>[2x]HHHHHHSSGLVPRGSHMQTTTVYSLEDLLPYLKQDNVDVKLAPGTYNVNGFDVGEDRLFSTTPLFLFEGSNSTYDFTDVKLNINTVVLTKFGNNEVNEIQILGNNNVLKNLKLEDIGTTAPSNRAQSIVIDGRDNRIEG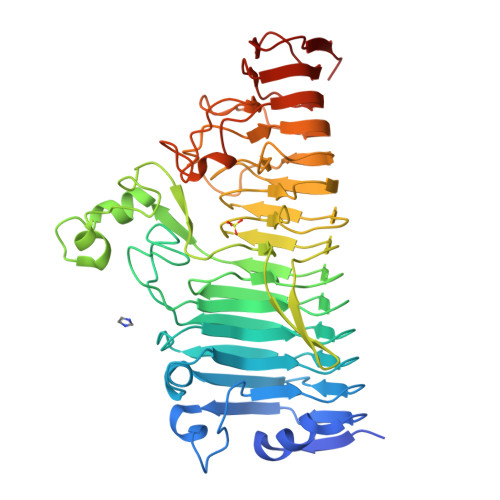FHLTIRGSYPYGYGDAFGKGGGSVINHRKHSGVLIRGLRNHLKDCTIISRSYGAIVFMQAASYPTVEGCYIEGEMRSTDDMLAEEGTGSPADKVDFMTVWGYKLPAGYMMSLQEGGIRAYNAGTTYIDGVEIQRATDNPTVLNCTIKNARTGVTLAHANGTKYVEGCTVLGCENGYSIGSGTVVNCGADAIYGPVFKNTYGSDKGYNADITILPPSDAYYNGHDAVAYIGGSNHNLTFRSEITEIPSNLKIMVSGDLQGLRVLHGSNPSQNNFAGTNIVLRNLTNFPVDLHSDSSNITVTSCDTDNITDNGTNNSIEAIDCDSD>MGAHSKEMAPLMGKRTTAPGGNPVVLTEKRPADLTPTKKSAHFFLEIEGFEPNPTVTKTSPPIFSKPMDSNIRQCLSGNCDDMDSPQSPQDDVTETPSNPNSPSANLAKEEQRQKKKRLKKRIFAAVSEGCVEELRELLQDLQDLCRRRRGLDVPDFLMHKLTASDTGKTCLMKALLNINPNTKEIVRILLAFAEENDILDRFINAEYTEEAYEGQTALNIAIERRQGDITAVLIAAGADVNAHAKGVFFNPKYQHEGFYFGETPLALAACTNQPEIVQLLMENEQTDITSQDSRGNNILHALVTVAEDFKTQNDFVKRMYDMILLRSGNWELETMRNNDGLTPLQLAAKMGKAEILKYILSREIKEKPLRSLSRKFTDWAYGPVSSSLYDLTNVDTTTDNSVLEIIVYNTNIDNRHEMLTLEPLHTLLHTKWKKFAKYMFFLSFCFYFFYNITLTLVSYYRPREDEDLPHPLALTHKMSWLQLLGRMFVLIWATCISVKEGIAIFLLRPSDLQSILSDAWFHFVFFVQAVLVILSVFLYLFAYKEYLACLVLAMALGWANMLYYTRGFQSMGMYSVMIQKVILHDVLKFLFVYILFLLGFGVALASLIEKCSKDKKDCSSYGSFSDAVLELFKLTIGLGDLNIQQNSTYPILFLFLLITYVILTFVLLLNMLIALMGETVENVSKESERIWRLQRARTILEFEKMLPEW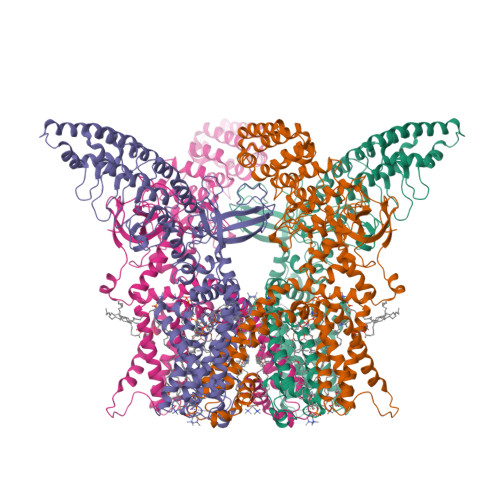LRSRFRMGELCKVADEDFRLCLRINEVKWTEWKTHVSFLNEDPGPIRRTADLNKIQDSSRSNSKTTLYAFDELDEFPETSVLVPRGSAAAWSHPQFEK[4x]>MHHHHHHSSGRENLYFQGIRMSQILEPRSEEDWTAHRTRIVCTMGPACWNVDTLVKMIDAGMNVCRLNFSHGDHETHARTVQNIQEAMKQRPEARLAILLDTKGPEIRTGFLKDHKPITLQQGATLKIVTDYNLIGDETTIACSYGALPQSVKPGNTILIADGSLSVKVVEVGSDYVITQAQNTATIGERKNMNLPNVKVQLPVIGEKDKHDILNFGIPMGCNFIAASFVQSADDVRYIRGLLGPRGRHIRIIPKIENVEGLVNFDEILAEADGIMIARGDLGMEIPPEKVFLAQKMMIAKCNVVGKPVITATQMLESMIKNPRPTRAEAADVANAVLD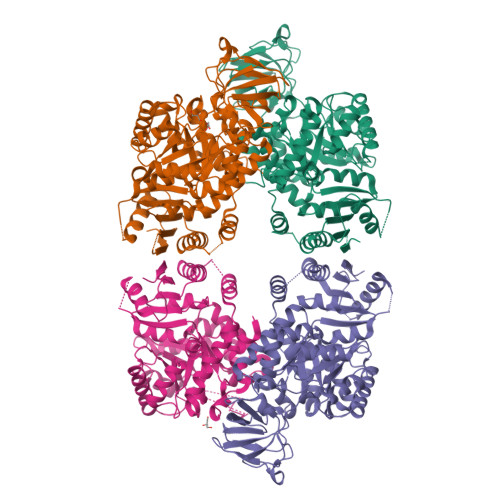GTDCVMLSGETANGEFPVITVETMARICYEAETCVDYPALYRAMCLAVPPPISTQEAVARAAVETAECVNAAIILALTETGQTARLIAKYRPMQPILALSASESTIKHLQVIRGVTTMQVPSFQGTDHVIRNAIVVAKERELVTEGESIVAVHGMKEEVAGSSNLLKVLTVE[4x]A major factor that limits the expansion of shrimp cultures is, however, infectious diseases from viruses, such as P. vannamei nodavirus (PvNV) and M. rosenbergii nodavirus (MrNV), which have inflicted heavy economic losses. The Nodaviridae genome comprises two single-stranded positive-sense RNA that encode the capsid protein for viral capsid assembly, the RNA polymerase for RNA replication, and the B2 protein for host RNA interference suppressor. While the shell domains (S-domains) of PvNV and MrNV contain conserved sequences of 62% identity, the protrusion domains (P-domains) and N-arms show low sequence identities of only 17% and 43%, respectively. In this work, we have determined the cryo-EM structures of T = 3 and T = 1 PvNV-LPs at atomic resolution, the crystal structures of the P-domains of PvNV and MrNV (PvNVPd and MrNVPd), and the crystal structure of the S-domain of PvNV (ΔN-ARM-PvNVSd) in the T = 1 subviral particle (SVP).

The structure of a virion-sized T = 3 PvNV-LP was determined by cryo-EM at 3.5 Å resolution. The cryo-EM map clearly shows T = 3 icosahedral symmetries with 90 spikes, composed of 180 copies of the 37-kDa full-length capsid proteins in total, distributed along the icosahedral 2-fold (I2) axes and the quasi 2-fold (Q2) axes on the surface. The icosahedral asymmetric unit (iASU) within the T = 3 PvNV-LP contains three capsid proteins occupying inequivalent sites with somewhat different conformations, which will be henceforth referred to as A–C subunits. The cryo-EM map allowed modeling of residues 64−368 for subunits A and B, and residues 31−368 for subunit C. Thus, the T = 3 shell exists as slightly different dimeric capsomeres consisting of an asymmetric A/B and a symmetric C/C dimers with the bent and flat conformations, respectively. In the T = 3 PvNV-LP, the ordered linkers from the C/C dimer exhibit a parallel structure at the opposite side, whereas the linkers from the A/B dimer adopt another new structural feature with a cross conformation. Remarkably, one iASU of the T = 3 PvNV-LP contains three sets of two Ca2+ ions, located at the interfaces between subunit pairs, which are coordinated with side chains of Asp146, Asp148 and Asp151 that form a 146DxDxxD151 motif at the E–F loop, Glu118 at the C–D loop, and Asn250 beside the linker from the neighboring subunit. Furthermore, residues 47–55 of the N-arms from subunits C5, C6, and C8 are engaged with hydrogen bonds to form a β-annulus structure around the I3 axis. Our cryo-EM map of the recombinant T = 3 PvNV-LP contain some information about the icosahedral-averaged endogenous RNA structure.

>[3x]MKRKPNSNQNNNNNRGNGNGLRRVRGGRVSRRRVVINQSNQSMPVTSNGAPLQALTSYSRPNVNKISRLGPDSDFLTSVVAKASTSIVTPADRILVKQPLSASSFPGTRITGLSSYWERYKWLSAVARYVPAVPNTVACQFVMYIDTDPLDDPSNISDDNQIVRQAVSQAGSNQFNFNTSKTVPLIVRADNQYYYTGVDKQNLRFSLQGILYIIQVTDLINFNGELITQDLTCGSLFLDWLVNFSIPQINPTSLTDVRVDKAVNFIKPEVSGVAEIQTVTGLSPSTSYLLTPAFLEQNFQSEAGIYILSATPVEGEGTISINMDPTVTTVSGFIKVKTDTFGTFDLSVVLTTASKKQTTGFNIIAATS> MDFYQLPGSPPCRAVALTAAALDIEMNFKQVNLMNGEHLKPEFLKINPQHTIPTIDDNGFRLWESRAIMTYLADQYGKND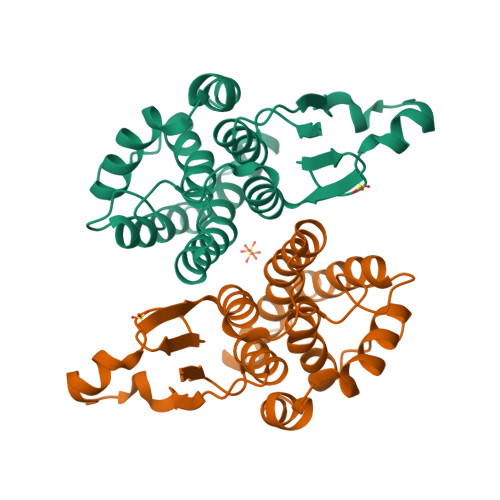TLYPKDLKKRAIVNQRLYFDLCSLYKSFMDYYYPIIFMKAVKDQAKYENIGTALSFLDKFLEGENYVAGKNMTLADLSIVSTVSTLEALDYDLSKYKNVTRWFAKIKPEIPKYEEYNNAGLKMFKELVNEKLSKK>MNSLFASTARGLEELLKTELENLGAVECQVVQGGVHFKGDTRLVYQSLMWSRLASRIMLPLGECKVYSDLDLYLGVQAINWTEMFNPGATFAVHFSGLNDTIRNSQYGAMKVKDAIVDAFTRKNLPRPNVDRDAPDIRVNVWLHKETASIALDLSGDGLHLRGYRDRAGIAPIKETLAAAIVMRSGWQPGTPLLDPMCGSGTLLIEAAMLATDRAPGLHRGRWGFSGWAQHDEAIWQEVKAEAQTRARKGLAEYSSHFYGSDSDARVIQRARTNARLAGIGELITFEVKDVAQLTNPLPKGPYGTVLSNPPYGERLDSEPALIALHSLLGRIMKNQFGGWNLSLFSASPDLLSCLQLRADKQYKAKNGPLDCVQKNYHVAESTPDSKPAMVAEDYTNRLRKNLKKFEKWARQEGIECYRLYDADLPEYNVAVDRYADWVVVQEYAPPKTIDAHKARQRLFDIIAATISVLGIAPNKLVLKTRERQKGKNQY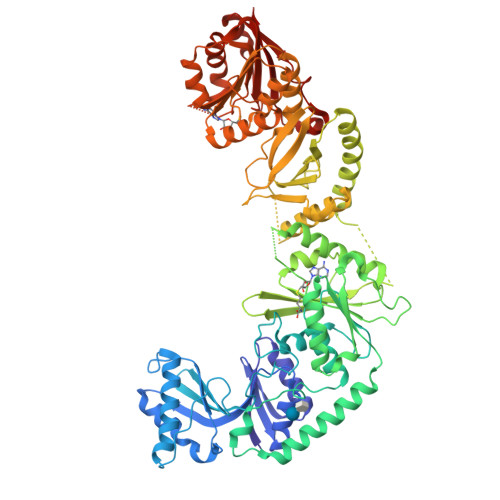QKLGEKGEFLEVTEYNAHLWVNLTDYLDTGLFLDHRIARRMLGQMSKGKDFLNLFSYTGSATVHAGLGGARSTTTVDMSRTYLEWAERNLRLNGLTGRAHRLIQADCLAWLREANEQFDLIFIDPPTFSNSKRMEDAFDVQRDHLALMKDLKRLLRAGGTIMFSNNKRGFRMDLDGLAKLGLKAQEITQKTLSQDFARNRQIHNCWLITAA[2x]>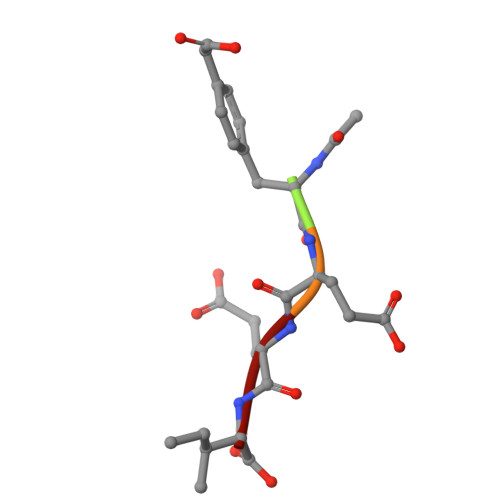 XFEEI> AMDKSAKAPQITIFDHRGCSRAPKESTGGKAGGQDDEMMVKVASTKVTVSESDAAKKLQEFITFEKGIDGPFTSKN;> AMDKSAKAPVITIFDHRGCSRAPKEYTGAKAGGKDDEMMVKAQSVKIEVSTGTAEGVLATSLAKMTK;>MLDAFSRVVTNADSKAAYVGGADLQALKKFISEGNKRLDSVNSIVSNASCIVSDAVSGMICENPSLISPSGNCYTNRRMAACLRDGEIILRYVSYALLSGDASVLEDRCLNGLKETYSSLGVPANSNARAVSIMKACAVAFVNNTASQKKLSTPQGDCSGL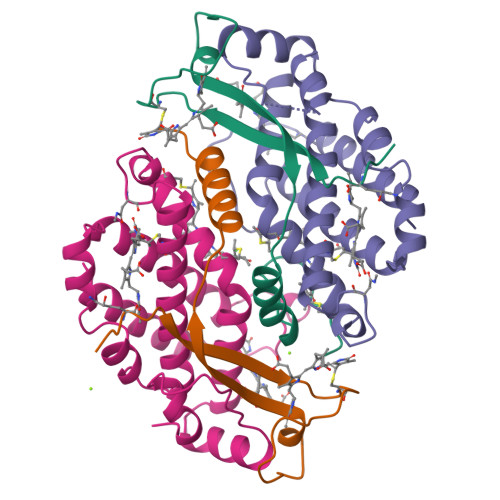ASEVGGYFDKVTAAIS[2x]> TENNDHINLKVAG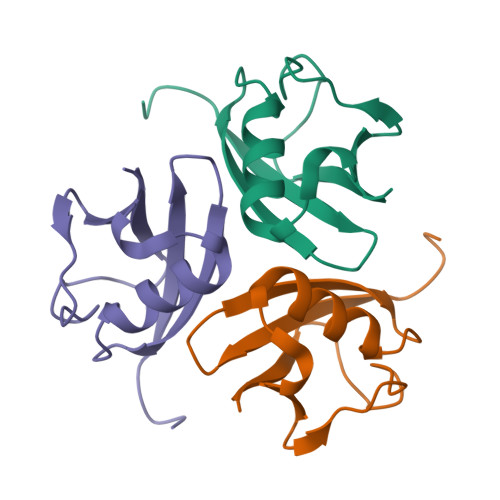QDGSVVQFKIKRHTPLSKLMKAYCERQGLSMRQIRFRFDGQPINETDTPAQLEMEDEDTIDVFQQ>[5x]NPGGFGNQGGFGNSRGGGAGLGNNQGSNMGGGMNFGAFSINPAMMA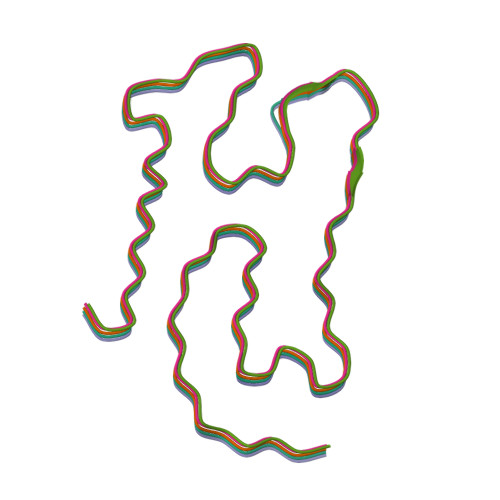AAQAALQSSWGMMGMLASQQNQSGPSGNNQNQGNMQ> PAPF;> AAQTNAPWGLARISSTSPGTSTYYYDESAGQGSCVYVIDTGIEASHPEFEGRAQMVKTYYYSSRDGNGHGTHCAGTVGSRTYGVVKKTQLFGV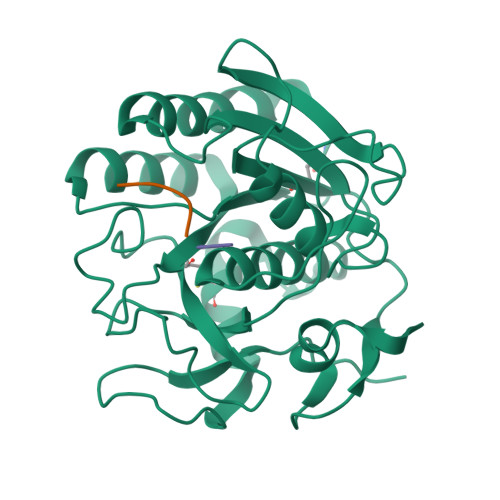KVLDDNGSGQYSTIIAGMDFVASDKNNRNCPKGVVASLSLGGGYSSSVNSAAARLQSSGVMVAVAAGNNNADARNYSPASEPSVCTVGASDRYDRRSSFSNYGSVLDIFGPGTSILSTWIGGSTRSISGTSMATPHVAGLAAYLMTLGKTTAASACRYIADTANKGDLSNIPFGTVNLLAYNNYQA GmPOPB is the macrocyclase responsible for macrocyclization of amatoxins, eight amino-acid ribosomal peptides with the core sequence IWGIGC(N/D)P. Amatoxins are cyclic peptides further modified by a characteristic sulfoxide cross-link between tryptophan and a cysteine, and hydroxylation (the extent of which vary). GmPOPB is an unusual enzyme catalyzing, depending on substrate length, proteolysis, or macrocyclization using the same catalytic machinery. The protein contains two domains as observed in other POP enzymes. The domain containing the putative catalytic residues (Ser577, Asp661, His698) comprises residues 1–81 and 450–728, and the other domain is a seven bladed β-propeller, comprising residues 82–449.

The same inactive mutant of GmPOPB was used to obtain a complex structure with the 25mer substrate; it comprises core (residues 1–8), linker, and recognition tag. Although we observed residual difference electron density for the N-terminal residues of the 25mer, we were unable to satisfactorily model it. In all 35mer and 25mer complexes, the enzyme adopts the same “closed” conformation in which the lid (the propeller domain) sits on top of the catalytic domain. There are no large differences between the protein backbone positions in the complexes with the 35mer and 25mer substrates (root mean square deviation (rmsd) of 0.48 Å over 720 Cα positions for the S577A structures). The recognition tail adopts an identical distorted 310 helix conformation inserted into the middle of the β-propeller domain in both the 25mer and 35mer complexes. The carboxyl terminus sits in a pocket where it makes water-mediated hydrogen bonds to the protein. To our surprise, there are only a few hydrogen bonds between the protein and the tail (Fig. 2c for the S577A–25mer complex and Fig. 2d for the S577A–35mer complex). Significant differences between the two substrates are observed for the residues of the linker region, since it occupies distinct conformations on the 25mer and 35mer complexes. The linker region, however, adopts very different arrangements in the two complexes, thus its interactions with the protein are quite distinct in the two structures. A comparison of the complex structures shows that in the 35mer complex there is disorder of side chains in the segment TAEHVD (linker region) but not in the 25mer.

>[2x]GMSSVTWAPGNYPSTRRSDHVDTYQSASKGEVPVPDPYQWLEESTDEVDKWTTAQADLAQSYLDQNADIQKLAEKFRASRNYAKFSAPTLLDDGHWYWFYNRGLQSQSVLYRSKEPALPDFSKGDDNVGDVFFDPNVLAADGSAGMVLCKFSPDGKFFAYAVSHLGGDYSTIYVRSTSSPLSQASVAQGVDGRLSDEVKWFKFSTIIWTKDSKGFLYQRYPARERHEGTRSDRNAMMCYHKVGTTQEEDIIVYQDNEHPEWIYGADTSEDGKYLYLYQFKDTSKKNLLWVAELDEDGVKSGIHWRKVVNEYAADYNIITNHGSLVYIKTNLNAPQYKVITIDLSKDEPEIRDFIPEEKDAKLAQVNCANEEYFVAIYKRNVKDEIYLYSKAGVQLTRLAPDFVGAASIANRQKQTHFFLTLSGFNTPGTIARYDFTAPETQRFSILRTTKVNELDPDDFESTQVWYESKDGTKIPMFIVRHKSTKFDGTAAAIQYGYGGFATSADPFFSPIILTFLQTYGAIFAVPSIRGGGEFGEEWHKGGRRETKVNTFDDFIAAAQFLVKNKYAAPGKVAINGAANGGLLVMGSIVRAPEGTFGAAVPEGGVADLLKFHKFTGGQAWISEYGNPSIPEEFDYIYPLSPVHNVRTDKVMPATLITVNIGDGRVVPMHSFKFIATLQHNVPQNPHPLLIKIDKSWLGHGMGKPTDKNVKDAADKWGFIARALGLELKTVE;>IWGIGCNPWTAEHVDQTLASGNDIC[2x]> MTTSAASQASLPRGRRTARPSGDDRELAILATAENLLEDRPLADISVDDLAKGAGISRPTFYFYFPSKEAVLLTLLDRVVNQADMALQTLAENPADTDRENMWRTGINVFFET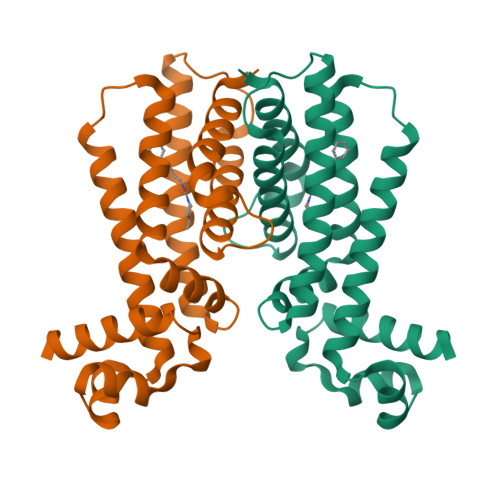FGSHKAVTRAGQAARATSVEVAELWSTFMQKWIAYTAAVIDAERDRGAAPRTLPAHELATALNLMNERTLFASFAGEQPSVPEARVLDTLVHIWVTSIYGENR> GPLGSMSDTALIFTLAWNVKQLAFDYTPNWGRGRPSSFIDTVTFPTVLT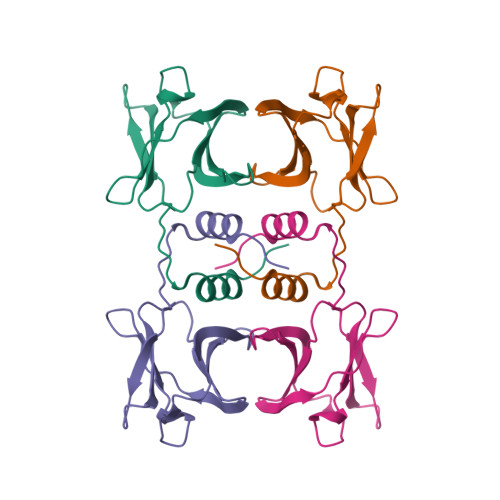DKAYTYRVVVSGKDLGVRPSYAVESDGSQKINFLEYNSGYGIADTNTIQVYVIDPDTGNNFIVAQWNYLEQKLISEEDLNSAVD6-(4-{[3-(2,6-dichlorophenyl)-5-(propan-2-yl)-1,2-oxazol-4-yl]methoxy}phenyl)-1-benzothiophene-3-carboxylic 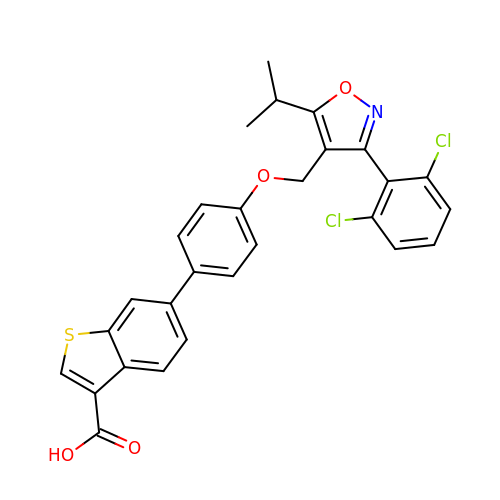acid | C28 H21 Cl2 N O4 S | UOKYTFQFOMGREX-UHFFFAOYSA-N> NAQVPTEEVSLEVLLSNGQKVLVNVLTSDQTEDVLEAVAAKLDLPDDLIGYFSLFLVREKEDGAFSFVRKLQEFELPYVSVTSLRSQEYKIVLRKSYWDSAYDDDVMENRVGLNLLYAQTVSDIERGWILVTKEQHRQLKSLQEKVSKKEFLRLAQTLRHYGYLRFDACVADFPEKDCPVVVSAGNSELSLQLRLPGQQLREGSFRVTRMRCWRVTSSVPLPSGSTSSPGRGRGEVRLELAFEYLMSKDRLQWVTITSPQAIMMSIC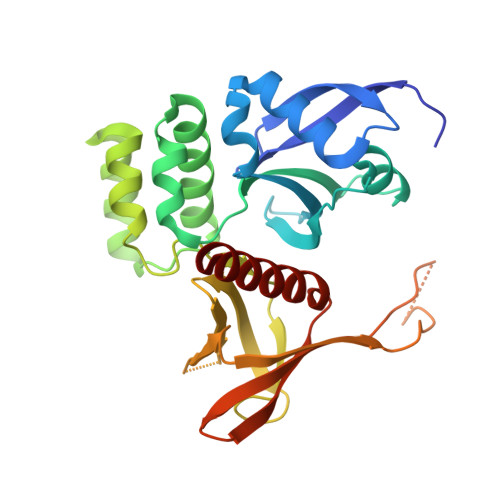LQSMVDELMVKKS> GSSSHSMRYFVTSVSEPGQQVPQFSYVGYVDDQEFVSYNASTRRYLPKVPWISKVEKNDPDYWERNTLYAQGHERSFRDHLATLAEYYNQSGGLHTFQWMYGCELRNDWSKGGYYQYAYDGRDYISLDKDTLTWMAADVPAQNTKRKWDADFRDNEYKKTYLEETCIEWLQRYLNYGKETLLRTEVPEVKVTRKEDYDGMETLICRVGGFYPKDIDIDWTRDGEVWLQDVFHGLVSPNSDGTYYTWRSVKVDPKERERYKCHVEHDGLPNPVDVAW;> TQKAPSVQVYFRHPAEKGKENTFHCYAESFHPPKINITLLKNGIPMENVQQSDLSFKKDWTFERLVYAKVIPDGKAEFACKVEHI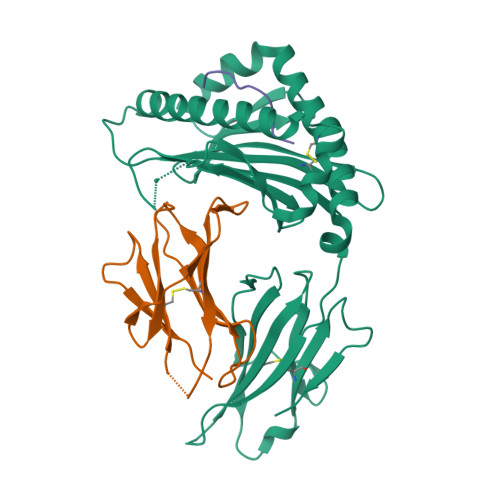TLPQPMIYKLDQEY;> HVYGPLKPI>[4x]EAEEDGDLQCLCVKTTSQVRPRHITSLEVIKAGPHCPTAQLIATL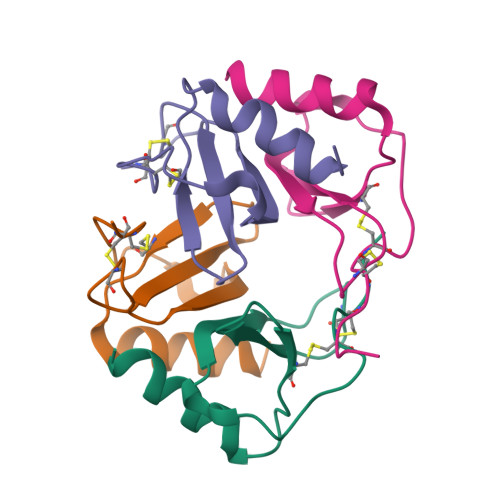KNGRKICLDLQAPLYKKIIKKLLES>EELPQIEIVQEGDNTTFAKPGDTVTIHYDGKLTNGKEFDSSRKRGKPFTCTVGVGQVIKGWDISLTNNYGKGGANLPKISKGTKAILTIPPNLAYGPRGIPGIIGPNETLVFEVELLGVNGQ[8x]

The 12-kDa FK506-binding protein (FKBP12) is a ubiquitously expressed peptidyl-prolyl isomerase with considerable homology between fungal pathogens and is thus a prime candidate for future targeting efforts to generate a panfungal strategy. PPIase proteins all catalyze the cis/trans isomerization of peptide bonds N terminal to proline residues in polypeptide chains. In addition to its role as a PPIase, FKBP12 is a member of the immunophilin family and is the target of the immunosuppressive drugs FK506 and rapamycin. Three extended loops, which have been called the 40s loop (between β2 and β3), the 50s loop (between β3′ and α1), and the 80s loop (between β4 and β5), surround a deep active-site pocket that binds both FK506 and rapamycin.

However, to confirm that this is indeed the catalytic pocket in the C. albicans protein, we next sought to determine the C. albicans FKBP12-FK506 structure. Interestingly, initial attempts to obtain crystals of the protein-FK506 complex failed, as the intermolecular interaction appeared to be strongly favored, leading to the production of the same apo crystal forms. Thus, we generated a P104G mutation in C. albicans FKBP12 and crystallized and obtained the apo FKBP12(P104G) structure to 2.0 Å. We next used the FKBP12(P104G) protein to obtain the structure bound to FK506. The structure revealed that, similar to other FKBP12-FK506 complexes, the immunosuppressant binds in the active-site pocket, surrounded by the 40s, 50s, and 80s loops. Comparison of this structure with the apo C. albicans structures with bound self-substrates revealed that the 80s loop that is inserted into the active site of the adjacent subunit binds in precisely the same location as the FK506 substrate/transition state homolog.>[2x]MDTEKLMKAGEIAKKVREKAIKLARPGMLLLELAESIEKMIMELGGKPA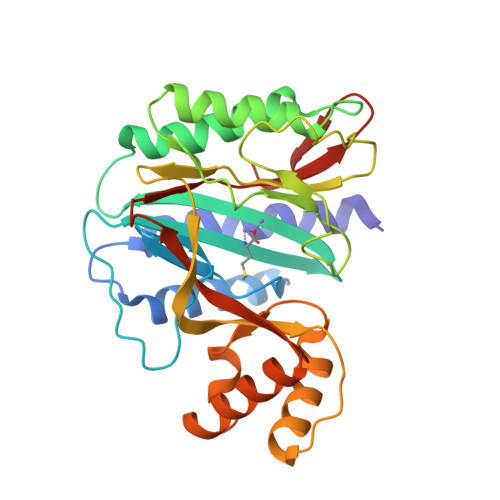FPVNLSINEIAAHYTPYKGDTTVLKEGDYLKIDVGVHIDGFIADTAVTVRVGMEEDELMEAAKEALNAAISVARAGVEIKELGKAIENEIRKRGFKPIVNLSGHKIERYKLHAGISIPNIYRPHDNYVLKEGDVFAIEPFATIGAGQVIEVPPTLIYMYVRDVPVRVAQARFLLAKIKREYGTLPFAYRWLQNDMPEGQLKLALKTLEKAGAIYGYPVLKEIRNGIVAQFEHTIIVEKDSVIVTTE>SNATRFERNFLINSLMFLETILSVDKKLDDAIHHFTQGQYENPRYQINSRITNADDWSKEDKLKFTSAIAEAIALVSEKYENPTSETTEQIQSARNILLDNYVPLLTANTDPENRLKSVRENSSQIRKEL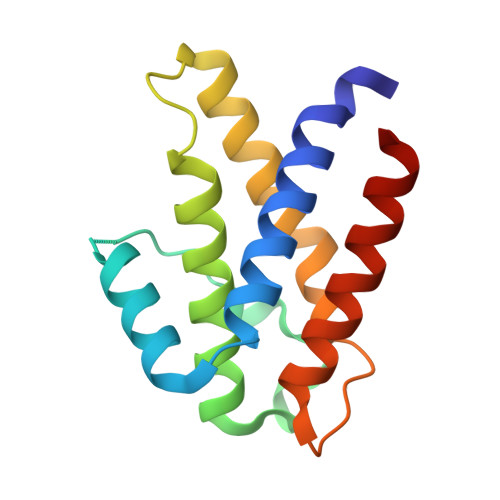IAKLKDE[3x]> GPLGSDLKDAEAVQKFFLEEIQLGEELLAQGDYEKGVDH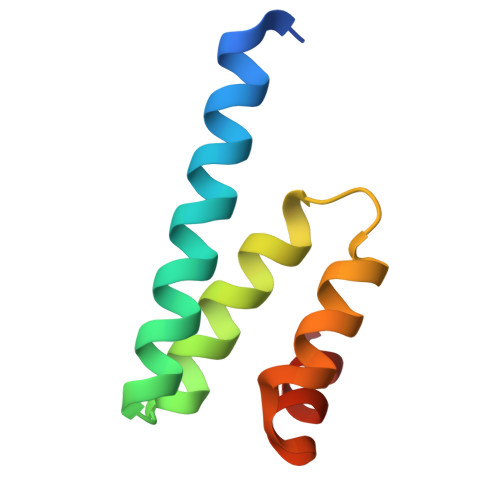LTNAIAVCGQPQQLLQVLQQTLPPPVFQMLLTKL>[2x]TYTTRQIGAKNTLEYKVYIEKDGKPVSAFHDIPLYADKENNIFNMVVEIPRWTNAKLEITKEETLNPIIQDTKKGKLRFVRNCFPHHGYIHNYGAFPQTWEDPNVSHPETKAVGDNDPIEVLEIGETIAYTGQVKQVKALGIMALLDEGETDWKVIAIDINDPLA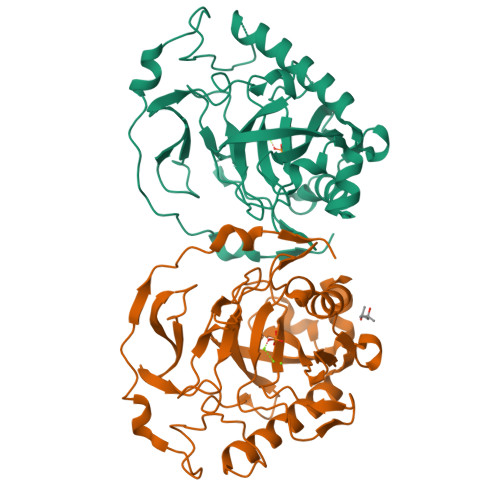PKLNDIEDVEKYFPGLLRATNEWFRIYKIPDGKPENQFAFSGEAKNKKYALDIIKETHDSWKQLIAGKSSDSKGIDLTNVTLPDTPTYSKAASDAIPPASLKADAPIDKSIDKWFFISGSV> MATPSFGNSSPQLTFTHVANFMNDAAADVSAVDAKQLAQIRQFLKANKTNLIESLNTIRQNVTSSGDHNKLRSTIANLLQINVDNDPFFAQSEDLSHAVEFFMSERSSRLHIVYSLLVNPDIDLETYSFIDNDRFNVVGKLISIISSVIQNYDIITASSLAHDYNNDQDMFTIVSLVQLKKFSDLKFILQILQILNLMILNTKVPVDIVNQWFLQYQNQFVEFCRNINSTDKSIDTSSLQLYKFQNFQDLSYLSETLISRISSLFTITTILILGLNTSIAQFDIQSPLYMDTETFDTVNSALENDVATNIVNEDPIFHPMIHYSWSFILYYRRALQSSESFDDSDITKFALFAESHDVLQKLNTLSEILSFDPVYTTVITVFLEFSLNFIPITASTSRVFAKIISKAPEQFIENFLTNDTFEKKLSIIKAKLPLLNESLIPLINLALIDTEFANFELKDICSFAVTKSSLNDLDYDLIADTITNSSSSSDIIVPDLIELKSDLLVAPPLENENSNCLLSIPKSTKGKILTIKQQQQQQQQQNGQQPPTTSNLIIFLYKFNGWSLVGRILQNLLHSYMEKGTQLDDLQHELMISIIKLVTNVVDPKTSIEKSSEILSYLSNSLDTSASTINGASIIQVIFEIFEISLQRKDYTSIVQCCEFMTMLTPNYLHLVSSYLNKSDLLDKYGKTGLSNMILGSVELSTGDYTFTIQLLKLTKVFIRESLSLKNIHISKRSKIDIINKLILHAIHIFESYYNWKYNNFLQKFEIAFHLTLIFYDVLHDVFTINPHQKDQLIISSSANKLLQLFLTPMDSIDLAPNTLTNILISPLNTTTKILGDKILGNLYSKVMNNSFKLCTLLIAIRGSNRDLKPSNLEKLLFINSSKLVDVYTLPSYVHFKVQIIELLSYLVEAPWNDDYPFLLSFLGEAKSMAFLKEVLSDLSSPVQDWNLLRSLYIFFTTLLESKQDGLSILFLTGQFASNKKINDESSIDKKSSILTVLQKNSLLLDSTPEEVSCKLLETITYVLNTWTNSKIFIKDPKFVNSLLAKLKDSKKLFQKKENLTRDETVSL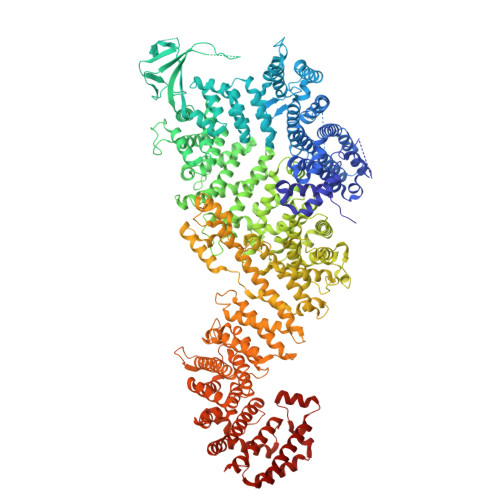IKKYKLISRIVEIFALCIYNSTDSNSEILNFLNQEDLFELVHHFFQIDGFNKTFHDELNLKFKEKWPSLELQSFQKIPLSRINENENFGYDIPLLDIVLKADRSWNEPSKSQTNFKEEITDASLNLQYVNYEISTAKAWGALITTFVKRSTVPLNDGFVDLVEHFLKLNIDFGSDKQMFTQIYLERIELSFYILYSFKLSGKLLKEEKIIELMNKIFTIFKSGEIDFIKNIGKSLKNNFYRPLLRSVLVLLELVSSGDRFIELISDQLLEFFELVFSKGVYLILSEILCQINKCSTRGLSTDHTTQIVNLEDNTQDLLLLLSLFKKITNVNPSKNFNVILASSLNEVGTLKVILNLYSSAHLIRINDEPILGQITLTFISELCSIEPIAAKLINSGLYSVLLESPLSVAIQQGDIKPEFSPRLHNIWSNGLLSIVLLLLSQFGIKVLPETCLFVSYFGKQIKSTIYNWGDNKLAVSSSLIKETNQLVLLQKMLNLLNYQELFIQPKNSDDQQEAVELVIGLDSEHDKKRLSAALSKFLTHPKYLNSRIIPTTLEEQQQLEDESSRLEFVKGISRDIKALQDSLFKDV>APLAQADTPSSPSIDQVEPYSSTAQVQFDEPEATGGVPILKYKAEWRAVGEEVWHSKWYDAKEASMEGIVTIVGLKPETTYAVRLAALNGKGLGEISAASEFKTQPVREPSAPKLEGQMGEDGNSIKVNLIKQDDGGSPIRHYLVRYRALSSEWKPEIRLPSGSDHVMLKSLDWNAEYEVYVVAENQQGKSKAAHFVFRTAAAH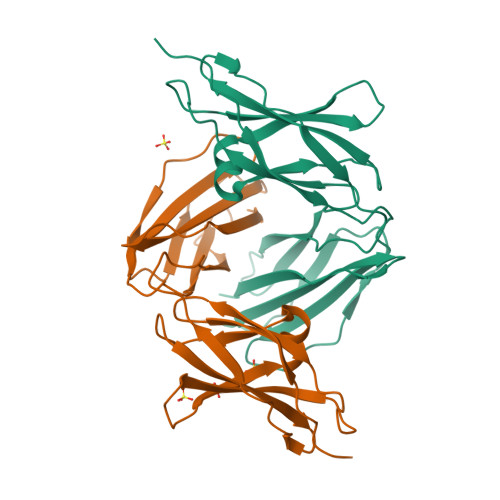HHHHH[2x]>[2x]MGSDKIHHHHHHMDALEIFKTLFSLVMRFSSYLPSNEEISDMK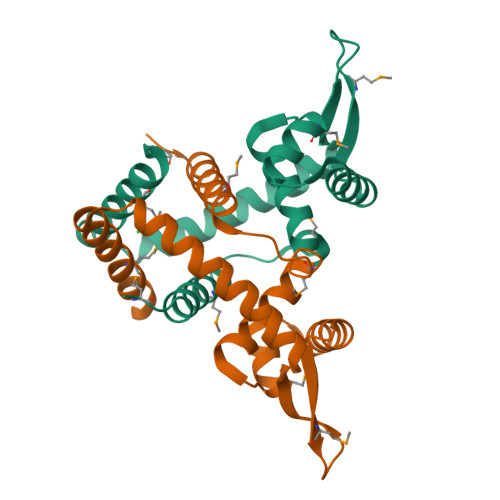TTELYAFLYVALFGPKKMKEIAEFLSTTKSNVTNVVDSLEKRGLVVREMDPVDRRTYRVVLTEKGKEIFGEILSNFESLLKSVLEKFSEEDFKVVSEGFNRMVEALSREGR>MRGSHHHHHHGSKDAVNYELIWSEWVKEAPAKEAANREEAVQRMRDCLKNNKTELRLKILGLTTIPAYIPEQITTLILDNNELKSLPENLQGNIKTLYANSNQLTSIPATLPDTIQEMELSINRITELPERLPSALQSLDLFHNKISCLPENLPEELRYLSVYDNSIRTLPAHLPSEITHLNVQSNSLTALPETLPPGLKTLEAGENALTSLPASLPPELQVLDVSKNQITVLPETLPPTITTLDVSRNALTNLPENLPAALQIMQASRNNLVRLPESLPHFRGEGPQPTRIIVEYNPFSERTIQNMQRLMSSVDYQGPRVLFAMGDFSIVRVTRPLHQAVQGWLTSLEEEDVNQWRAFEAEANAAAFSGFLDYLGDTQNTRHPDFKEQVSAWLMRLAEDSALRETVFIIAMNATISCEDRVTLAYHQMQEATLVHDAERGAFDSHLAELIMAGREIFRLEQIESLAREKVKRLFFIDEVEVFLGFQNQLRESLSLTTMTRDMRFYNVSGITESDLDEAEIRIKMAENRDFHKWFALWGPWHKVLERIAPEEWREMMAKRDECIETDEYQSRVNAELEDLRIADDSDAERTTEVQMDAERAIGIKIMEEINQTLFTEIMENILLKKEVSSLMSAYWR[2x];>MRGSHHHHHHGSMVKQIESKTAFQEALDAAGDKLVVVDFSATWCGPCKMIKPFFHSLSEKYSNVIFLEVDVDDCQDVASECE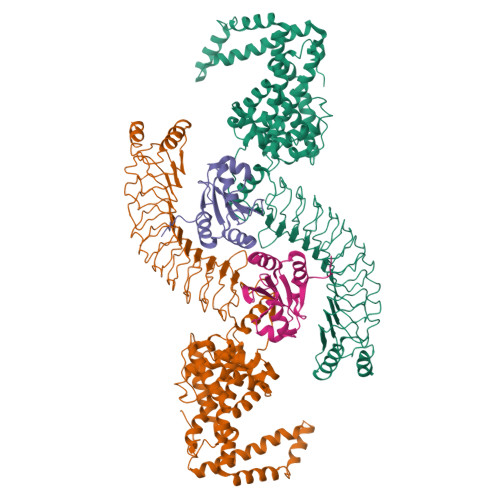VKCMPTFQFFKKGQKVGEFSGANKEKLEATINELV[2x]2-hydroxypropane-1,3-diyl dibutanoate | C11 H20 O5 | 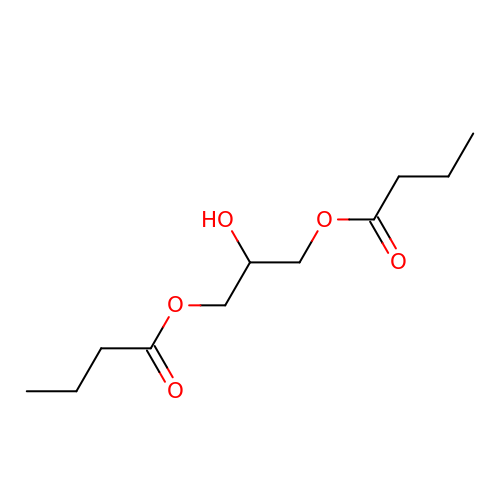KBWFWZJNPVZRRG-UHFFFAOYSA-N5'-O-[(S)-hydroxy(4-methyl-1H-imidazol-5-yl)phosphoryl]guanosine 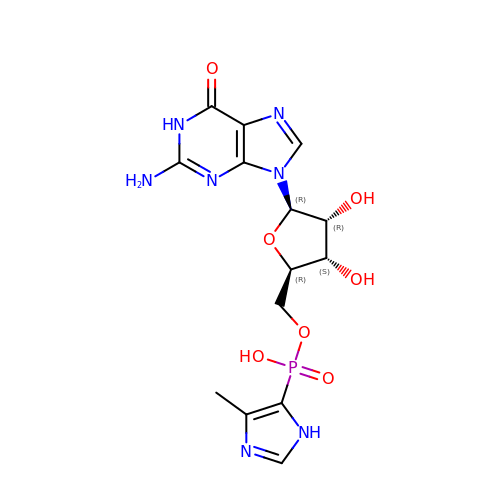| C14 H18 N7 O7 P | MUFMHNGPMISZRD-HTVVRFAVSA-N>GSKDKKEAGADSKTIKLWVPTGSKKSYADTIAKFEKDSGYTVKVVESEDPKAQEKIKKDASTAADVFSLPHDQLGQLVESGTIQEVPEKYNKEIAATSTDQALIGAQYKGKTYAFPFGIESQVLFYNKSKLAAEDVTSYDTITTKATFGGTFKQANSYATGPLFMSVGNTLFGENGEDVKGTNWGNEKGAAVLKWIADQASNKGFVSLDANNVISKFGDGSVASFESGPWDYEAAQKAIGKENLGVAIYPKVTIGGETVQQKAFLGVKLYAVNQAPAKGDTKRIAASYKLASYLTNAESQENQFKTR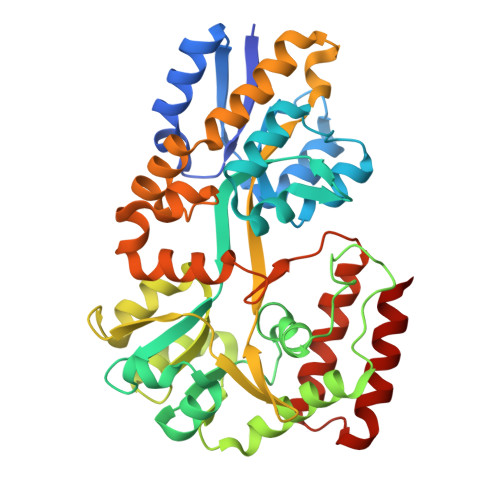NIVPANKEVQSSEAVQSNELAKTVITMGSSSDYTVVMPKLSQMGTFWTESAAILSDAFNGKIKESDYLTKLQQFDKDIAATK[2x]>MKTFEILKHLQADAIVLFMKVHNFHWNVKGTDFFNVHKATEEIYEEFADMFDDLAERIVQLGHHPLVTLSEAIKLTRVKEETKTSFHSKDIFKEILEDYKYLEKEFKELSNTAEKEGDKVTVTY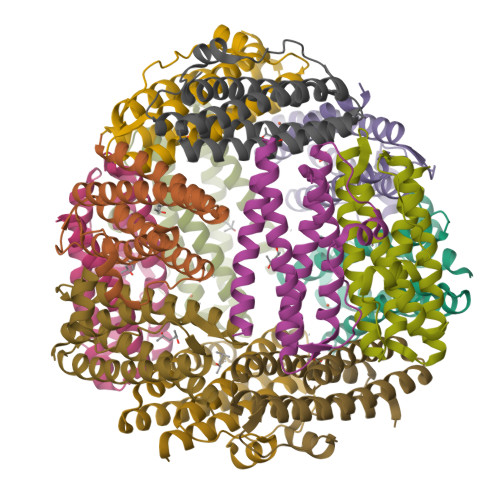ADDQLAKLQKSIWMLQAHLA[12x]> MSAGKLPEGWVIAPVSTVTTLIRGVTYKKEQAINYLKDDYLPLIRANNIQNGKFDTTDLVFVPKNLVKESQKISPEDIVIAMSSGSKSVVGKSAHQHLPFECSFGAFCGVLRPEKLIFSGFIAHFTKSSLYRNKISSLSAGANINNIKPASFDLINIPIPPLAEQKIIAEKLDTLLAQVDSTKARFEQIPQILKRFRQAVLGGAVNGKLTEKWRNFEPQHSVFKKLNFESILTELRNGLSSKPNESGVGHPILRISSVRAGHVDQNDIRFLECSESELNRHKLQDGDLLFTRYNGSLEFVGVCGLLKKLQHQNLLYPDKLIRARLTKDALPEYIEIFFSSPSARNAMMNCVKTTSGQKGISGKDIKSQVVLLPPVKEQAEIVRRVEQLFAYADTIEKQVNNALARVNNLTQSILAKAFRGELTAQWRAENPDLISGENSAAALLEKIKAERAASGGKKASRKKS;>MNNNDLVAKLWKLCDNLRDGGVSYQNYVNELASLLFLKMCKETGQE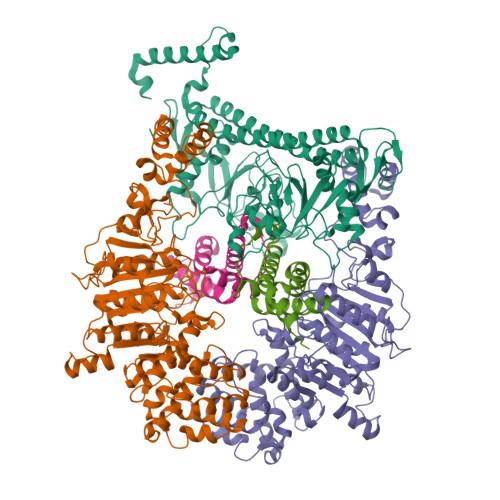AEYLPEGYRWDDLKSRIGQEQLQFYRKMLVHLGEDDKKLVQAVFHNVSTTITEPKQITALVSNMDSLDWYNGAHGKSRDDFGDMYEGLLQKNANETKSGAGQYFTPRPLIKTIIHLLKPQPREVVQDPAAGTAGFLIEADRYVKSQTNDLDDLDGDTQDFQIHRAFIGLELVPGTRRLALMNCLLHDIEGNLDHGGAIRLGNTLGSDGENLPKAHIVATNPPFGSAAGTNITRTFVHPTSNKQLCFMQHIIETLHPGGRAAVVVPDNVLFEGGKGTDIRRDLMDKCHLHTILRLPTGIFYAQGVKTNVLFFTKGTVANPNQDKNCTDDVWVYDLRTNMPSFGKRTPFTDEHLQPFERVYGEDPHGLSPRTEGEWSFNAEETEVADSEENKNTDQHLATSRWRKFSREWIRTAKSDSLDISWLKDKDSIDADSLPEPDVLAAEAMGELVQALSELDALMRELGASDEADLQRQLLEEAFGGVKE[2x];>MAMSNMTYNNVFDHAYEMLKENIRYDDIRDTDDLHDAIHMAADNAVPHYYADIFSVMASEGIDLEFEDSGLMPDTKDVIRILQARIYEQLTIDLWEDAEDLLNEYLEEVEEYEEDE[2x]>[7x]GPHMRKQEIIKTTEQLIEAVNNGDFEAYAKICDPGLTSFEPEALGNLVEGMDFHRFYFENLLAKNSKPIHTTILNPHVHVIGEDAACIAYIRLTQY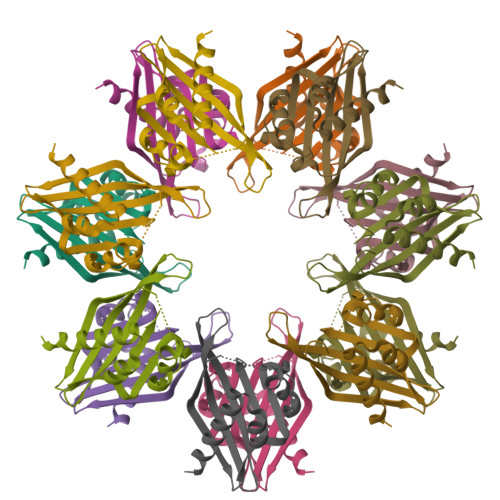IDGQGRPRTSQSEETRVWHRRDGKWQNVHFHCSGAPVAPLQ methyl 5-acetamido-3,5,9-trideoxy-9-[(phenylcarbonyl)amino]-D-glycero-alpha-D-galacto-non-2-ulopyranosidonic acid | C19 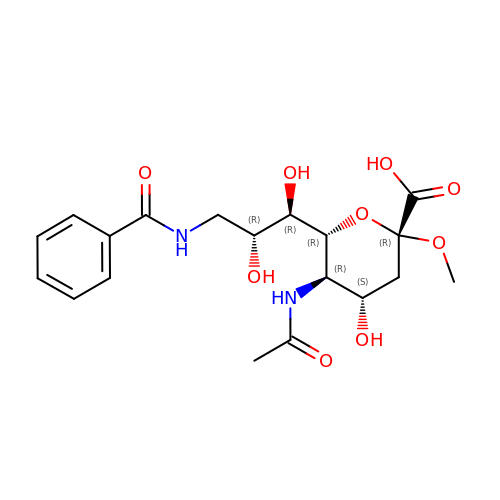H26 N2 O9 | ULZLCALWUIQOMB-YRIWUQCMSA-N>[6x]MLPRPSGTYAGLPIADYGDAPPLSTKTMFWRTSPEKLPPGAWEPAYLGSKDERVDGPSLQQVMRDQLKPYSEPRGLLPPQEILDAVCDAIENRLENTLEPQKPWTFKKACESLDKNTSSGYPYHKQKSKDWTGSAFIGDLGDQATHANNMYEMGKSMRPIYTAALKDELVKPDKIYGKIKKRLLWGSDLGTMIRAARAFGPFCDALKETCIFNPIRVGMSMNEDGPFIFARHANFRYHMDADYTRWDSTQQRAILKRAGDIMVRLSPEPDLARVVMDDLLAPSLLDVGDYKIVVEEGLPSGCPCTTQLNSLAHWILTLCAMVEVTRVDPDIVMQESEFSFYGDDEVVSTNLELDMVKYTMALRRYGLLPTRADKEEGPLERRQTLQGISFLRRAIVGDQFGWYGRLDRASIDRQLLWTKGPNHQNPFETLPGHAQRPSQLMALLGEAAMHGEKYYRTVASRVSKEAAQSGIEMVVPRHRSVLRWVRFGTMDAETPQERSAVFVNEDAAALEHHHHHH

Norovirus (NoV) is a positive-sense single-stranded RNA (+RNA) virus belonging to the Caliciviridae family. ORF1 encodes a polyprotein that is cleaved into non-structural proteins, including virion protein genome-linked (VPg) and RNA-dependent RNA polymerase (RdRp). VPg covalently attached to the 5′ end of viral RNAs plays crucial roles in viral protein translation and genome replication. Moreover, the crystal structure of the complex provided the evidence that the interaction between VPg and RdRp plays a crucial role in NoV replication through the higher-order multimer formation of RdRp molecules.

Next, we determined the complex structure of RdRp-VPg(1-73) at 3.1 Å resolution. Continuous electron density was observed at the base of the palm domain of RdRp in the initial map. Two helix backbones (α1 and α2) modeled for VPg were fitted to the electron density with lower B factor, which was verified by examining a simulated annealing composite omit map at the 1.2σ level. However, the electron densities for the side chains of VPg were not well defined, whereas those of RdRp were clearly interpretable. MNV VPg had a distinct helix-loop-helix conformation and bound to the palm domain of RdRp, and the binding site was relatively similar to that of EV71 RdRp but far from that of VPg at the active site of FMDV or the thumb domain of CV RdRps. The electron density for the oligo(A)8 RNA was not visible in the complex structure, despite the presence of the oligonucleotide in the crystallization solution. A large ball-like hexameric arrangement of RdRp was observed in the crystal structures. A face-to-face contact of the palm domains was capable of forming a dimeric structure, and the trimer interface was largely made up of the thumb and fingers domains in the hexameric complex. The crystal structure of the MNV RdRp-VPg(1-73) complex showed a more tightly packed arrangement of RdRp molecules than that of RdRp molecules themselves; a hexamer of RdRp molecules was surrounded compactly by six neighboring hexamers and this was mediated by specific binding of VPg(1-73). Further, the interactions between RdRp molecules in the RdRp-VPg(1-73) complex were distinct from that of the native; interactions between Arg329 and Gln389 and between Asp91 and Arg411 of adjacent RdRp molecules were observed in the RdRp-VPg(1-73) complex structure but absent in the native.> MSQRIIQPSASDQQFPGKSDGYEYTVGPKQAITSEASTTYIPSRIYSESLLFKRQEASLSAMAFLFQEMISQLHRTCKTAGDFETKLSDYGHNIGIRLLELLNFRASVSPSSLPRASAFLSQNESSSKLSNASNSPGMLANSSTATSASANERLQEKQTESLSNYITKMRRRDLKILDILQFIHGTLWSYLFNHVSDDLVKSSERDNEYMIVDNFPTLTQFIPGENVSCEYFVCGIIKGFLFNAGFPCGVTAHRMPQ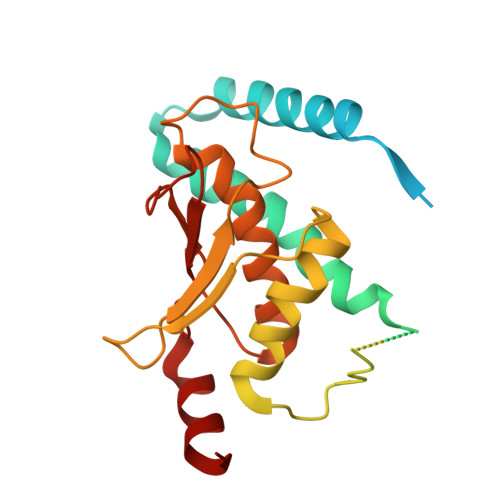GGHSQRTVYLIQFDRQVLDREGLRFG> MHHHHHHQIGWRREGIKYRR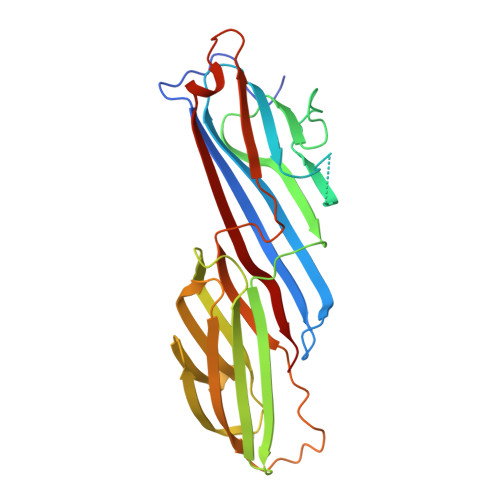NELFLDVLESVNLLMSPQGQVLSAHVSGRVVMKSYLSGMPECKFGMNDKIVIEKQGKGTADETSKSGKQSIAIDDCTFHQCVRLSKFDSERSISFIPPDGEFELMRYRTTKDIILPFRVIPLVREVGRTKLEVKVVIKSNFKPSLLAQKIEVRIPTPLNTSGVQVICMKGKAKYKASENAIVWKIKRMAGMKESQISAEIELLPTNDKKKWARPPISMNFEVPFAPSGLKVRYLKVFEPKLNYSDHDVIKWVRYIGRSGIYETRC Here structural analysis of hydroxyketoacid aldolase from Sphingomonas wittichii RW1 (SwHKA) revealed a dynamic movement of the metal cofactor between two coordination spheres without protein scaffold rearrangements. Holo‐SwHKA forms a trimer of homodimers, in which each monomer adopts an (α/β)8 triosephosphate isomerase (TIM) barrel fold. In total, holo‐SwHKA contains six equivalent active sites; each of which is formed from amino acids from two different domain‐swapped dimers. The transition from M2+ R to M2+ A,S is induced by bidentate substrate binding and occurs without a concomitant rearrangement of the protein scaffold.

To gain insight into the earlier observed activation of the enzyme by phosphate and a possible interaction thereof with the metal, phosphate was included into the crystallisation and soaking studies. Neither was the case for SwHKA. Docking studies did however reveal a potential docking site, close to H44 (Figure S6a&b). The docking does however support the earlier proposed function in the pyruvate deprotonation, studied by H/D exchange. In both cases 100–300 fold improved deprotonation rates were observed. This could be enabled by a phosphate in concert with H44. In the presence of ketoacids, bidentate substrate coordination affords M2+ A,S as the lowest energy complex and predominant state in crystal structures. Bidentate substrate coordination therefore seems to constitute the driving force for the transition of the metal cofactor from M2+ R via M2+ A,W into the catalytically active configuration M2+ A,S.

>HNKVRTCWNEGRPALAGWLQLPGTLHAEALARLDYDAVVIDMQASPIDFGQVAPMLIAIELGGAEPFVRTQVNDPSDIMKLLDAGAYGIIAPMVNTRAEAQTLASALHYSPRGLRSFGPRRPSLRYGSGYLAQASETVVGLAMIETREALANIDEILSVDGIDGVFIGPTDLALDLGHAPLVDTEEAEVVSAIAHVRERAHAAGKRVGIFCGSGGFARVKLAEGFDFVTAAPDLAMLSAAARQVIADARAL[2x]> SEQNTPLGGCILADTPITFNENKPVTKVKVRNTGDRPIQVGSHFHFFEVNRALEFDRAAAYGKRLNISSTTAIRFEPGDETEVPLIPFGGKQTLYGFNNLVDGWTGEGVVPNSERPDKL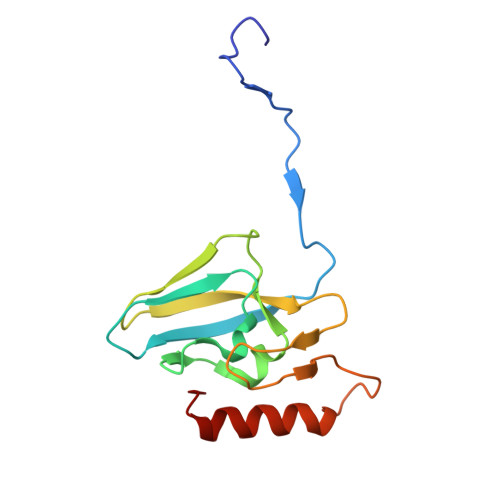EAIRRAAERGFKS> IKDILRRPVLLFNHVELDPDYTGFFIPIMPPSRMMQYKSGDKETSFQRLIGRTPQAAIMNLFRFWRGSLRYTIIIHSTDGHPIYVTHVPHTGNRVYGLMKVNNLHEYTKVPIFGCGLTTEMIIPSVNPSICVEVPFDTENNWAVTFDEDAQRNYSWRDKGDTVTGHLVVTPVVSVYMSVWVEAGDDFEVSNFYGPPSVKTNDWNYAFSDEH;> WMPINSIRVTVNGKRNDLLAQYYIPEDFLSTHAKCAPNTIPFETYVYGKYELEMKFVANGNKFQCGKVIISVKFDSYQADNINTGFQAALSRPHIMLDLSTNNEGVLKIPFRYHRAFVRNQTHKTATAGVRPGKFASIYVQVLSPLQTGEGGANDMFIRPFYRYTRAEFAGMSYKVPLT;> DEPRTTLDIARIWGLRSTFNWGSGDEHGKELFNTVLDPGLRFYDQDYEGQITPMEYVTGLYNFWSGPIELRFDFVSNAFHTGTVIISAEYNRSSTNTDECQSHSTYTKTFHLGEQKSVHFTVPYIYDTVVRRNTASAYLPVTDYD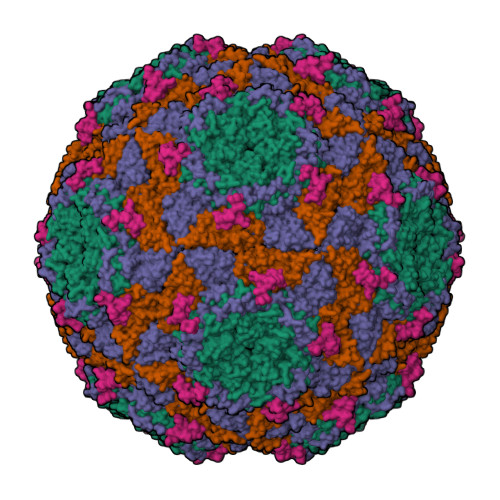KVDNVSRAQAMGIRAESKMRVKVRVVNVLRPVASTTSTIEVLVYMRGGKNYALHGLKQSTYWPSNSVVPIDSFPPDGYDP;> DNPHRFLPANVSNRWNEYSSAYLPRV> MRTTKKIVSAVLAACMLASTAVVSSFAATADDSSAVSSDYARDNSYTKAAEDIDAQYAYSGNDLGVTYTKDATTFKVWSPTATGVKLNIFTKGSDDEQGASKVASYTLEKMLVDGEWNGVWTITLVGEWKDYYYTYSVTTTDTTHIGSDATKTYETQDVYSTATGVNGKRSMIVDLDETDPEGWSNDSHVLLDKSTKSSVWELHIKDFSYDKASGVSDANRGKYLAFTENGTTLNGEGKVSTCIDYLKELGVTTVQLNPFYDFQSVNEAGDDSQFNWGYDPVNYNVPEGSYSSNPYDGKVRIKECKEMIKALHDAGISVVMDVVYNHTYSTDSCFQYTVPNYYYRMKTTGAFSDGSGCGNEGATERAMYRQYVIDSLKYWVNEYHVDGFRFALMGLMDVETMNMAREALDQIDPRITM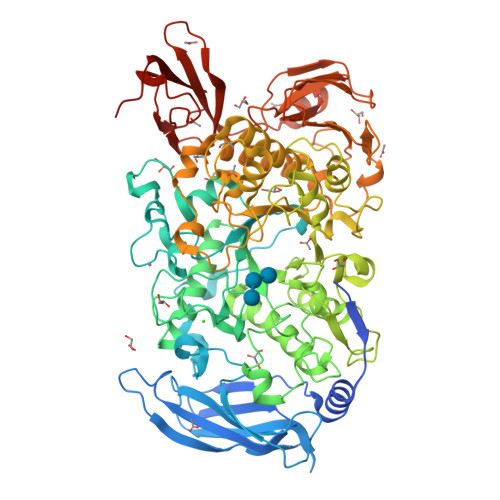WGEGWAGGDSYHPTNTCSGTKFYPATQANASRLSDRIAIFNDGIRDGIKGSAMDISDVGFIQGSKSSAKGVSYGVRANSSGTYKWKAQAPSQCVTYDACHDNATLYDQIIASTGLADYGERNSEAVKMNRLASAIIYTSQGISFTLAGEEMARSKDGDTNSYKSAANLNMIKWQNVVDYADVVSYYKGMMQIKSAFSPLTAMDNSYADKYTFTKKVSASTNQISFTIQNDVEGEWNKMAVIYNNATTAADVTLSDTSVTDWVVIANGETAGLDSLGEVTGSTFTVPARSAIVAVDKAGYESAGIHSSKGKVKVNYVYEATGEKLEDSVILQGSVGSGYVTVPSAVIPDTYIVSRIGGNAEGKYTSDMQEVTYYYTDYIPESL> GSHMASSIEFVRIDDRLVHGQVVTT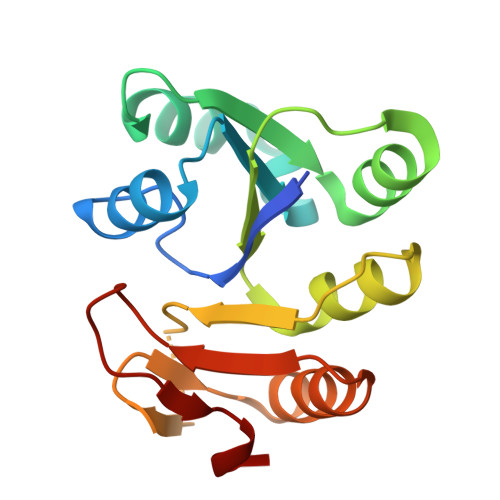WLKKYDIEQVIIVNDRISEDKTRQSILKISAPVGLKIVFFSVKRFVEVLNSVPIKKRTMLIYTNPKDVYDSIEGNLKLEYLNVGQMSKTEENEKVTGGVALGEEDKYYFKKIVDKGTRVEIQMVPNDKVTMLEKFL>GAMGSMRLLVSCVDSGSIKEVLCNIGTDTSVQSALQPFHVAPHLAEGLKAYVDRMWVISEDEAILARNSGVVELVKISKHLKENEALQVDPKGESKNEKSLSDDLPKFDISEFEITSSVSDLFDDAKLESLSSKSVKRTKLVDGFVTLCPIKKDSSNNTFVAATKSGLLHIIKKGEDKKLIKLASLGLKAPVEFLQLYDLEDTDTDKYIFAYGGEENLIKLVEIDSSFQSLKQIWEAKNVKNDRLDMRVPVWPMALRFLEPSPGKTEKGKLNYQFAAITRWSHLTKYSTQHGRKPFAQIDLLPNREPLSQMEVFDAKGENVVSSLGNFQSETFNELNVITTDYKKNVFKFDGNGRMLGKVGRDDITGSSTYIHVHDGKYLLQGGLDRYVRIFDIKTNKMLVKVYVGSRINFIVMLDDVEIEMPL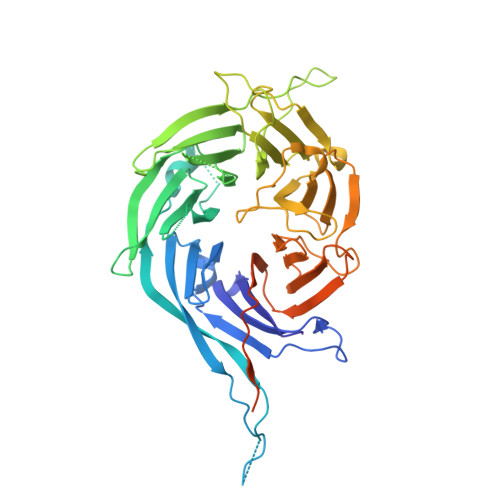SPSAKAAKGKQKRKVTELEEDADELWNKLEGKVAASKASKKSKI[2x]>[6x]MAAPARDPPGYRYAAAMVPTGSILSTIEVASHRRLFDFFAAVRSDENSLYDVEFDALLGSYCNTLSLVRFLELGLSVACVCTKFPELAYMNEGRVQFEVHQPLIARDGPHPVEQPVHNYMTKVIDRRALNAAFSLATEAIALLTGEALDGTGISLHRQLRAIQQLARNVQAVLGAFERGTADQMLHVLLEKAPPLALLLPMQRYLDNGRLATRVARATLVAELKRSFCDTSFFLGKAGHRREAIEAWLVDLTTATQPSVAVPRLTHADTRGRPVDGVLVTTAAIKQRLLQSFLKVEDTEADVPVTYGEMVLNGANLVTALVMGKAVRSLDDVGRHLLDMQEEQLEANRETLDELESAPQTTRVRADLVAIGDRLVFLEALEKRIYAATNVPYPLVGAMDLTFVLPLGLFNPAMERFAAHAGDLVPAPGHPEPRAFPPRQLFFWGKDHQVLRLSMENAVGTVCHPSLMNIDAAVGGVNHDPVEAANPYGAYVAAPAGPGADMQQRFLNAWRQRLAHGRVRWVAECQMTAEQFMQPDNANLALELHPAFDFFAGVADVELPGGEVPPAGPGAIQATWRVVNGNLPLALCPVAFRDARGLELGVGRHAMAPATIAAVRGAFEDRSYPAVFYLLQAAIHGNEHVFCALARLVTQCITSYWNNTRCAAFVNDYSLVSYIVTYLGGDLPEECMAVYRDLVAHVEALAQLVDDFTLPGPELGGQAQAELNHLMRDPALLPPLVWDCDGLMRHAALDRHRDCRIDAGGHEPVYAAACNVATADFNRNDGRLLHNTQARAADAADDRPHRPADWTVHHKIYYYVLVPAFSRGRCCTAGVRFDRVYATLQNMVVPEIAPGEECPSDPVTDPAHPLHPANLVANTVKRMFHNGRVVVDGPAMLTLQVLAHNMAERTTALLCSAAPDAGANTASTANMRIFDGALHAGVLLMAPQHLDHTIQNGEYFYVLPVHALFAGADHVANAPNFPPALRDLARHVPLVPPALGANYFSSIRQPVVQHARESAAGENALTYALMAGYFKMSPVALYHQLKTGLHPGFGFTVVRQDRFVTENVLFSERASEAYFLGQLQVARHETGGGVNFTLTQPRGNVDLGVGYTAVAATGTVRNPVTDMGNLPQNFYLGRGAPPLLDNAAAVYLRNAVVAGNRLGPAQPLPVFGCAQVPRRAGMDHGQDAVCEFIATPVATDINYFRRPCNPRGRAAGGVYAGDKEGDVIALMYDHGQSDPARPFAATANPWASQRFSYGDLLYNGAYHLNGASPVLSPCFKFFTAADITAKHRCLERLIVETGSAVSTATAASDVQFKRPPGCRELVEDPCGLFQEAYPITCASDPALLRSARDGEAHARETHFTQYLIYDASPLKGLSL;>[6x]MAAPQFHRPSTITADNVRALGTRGLVLATNNAQFIMDNSYPHPHGTQGAVREFLRGQAAALTDLGVTHANNTFAPQPMFAGDAAAEWLRPSFGLKRTYSPFVVRDPKTPSTP;>MITDCFEADIAIPSGISRPDAAALQRCEGRVVFLPTIRRQLALADVAHESFVSGGVSPDTLGLLLAYRRRFPAVITRVLPTRIVACPVDLGLTHAGTVNLRNTSPVDLCNGDPVSLVPPVFEGQATDVRLESLDLTLRFPVPLPTPLAREIVARLVARGIRDLNPDPRTPGELPDLNVLYYNGARLSLVADVQQLASVNTELRSLVLNMVYSITEGTTLILTLIPRLLALSAQDGYVNALLQMQSVTREAAQLIHPEAPMLMQDGERRLPLYEALVAWLAHAGQLGDILALAPAVRVCTFDGAAVVQSGDMAPVIRYP[2x];> MKTKPLPTAPMAWAESAVETTTSPRELAGHAPLRRVLRPPIARRDGPVLLGDRAPRRTASTMWLLGIDPAESSPGTRATRDDTEQAVDKILRGARRAGGLTVPGAPRYHLTRQVTLTDLCQPNAERAGALLLALRHPTDLPHLARHRAPPGRQTERLAEAWGQLLEASALGSGRAESGCARAGLVSFNFLVAACAAAYDARDAAEAVRAHITTNYGGTRAGARLDRFSECLRAMVHTHVFPHEVMRFFGGLVSWVTQDELASVTAVCSGPQEATHTGHPGRPRSAVTIPACAFVDLDAELCLGGPGAAFLYLVFTYRQCRDQELCCVYVVKSQLPPRGLEAALERLFGRLRITNTIHGAEDMTPPPPNRNVDFPLAVLAASSQSPRCSASQVTNPQFVDRLYRWQPDLRGRPTARTCTYAAFAELGVMPDDSPRCLHRTERFGAVGVPVVILEGVVWRPGGWRACA;> MNAHFANEVQYDLTRDPSSPASLIHVIISSECLAAAGVPLSALVRGRPDGGAAANFRVETQTRAHATGDCTPWRSAFAAYVPADAVGAILAPVIPAHPDLLPRVPSAGGLFVSLPVACDAQGVYDPYTVAALRLAWGPWATCARVLLFSYDELVPPNTRYAADGARLMRLCRHFCRYVARLGAAAPAAATEAAAHLSLGMGESGTPTPQASSVSGGAGPAVVGTPDPPISPEEQLTAPGGDTATAEDVSITQENEEILALVQRAVQDVTRRHPVRARPKHAASGVASGLRQGALVHQAVSGGALGASDAEAVLAGLEPPGGGRFASRGGPRAAGEDVLNDVLTLVPGTAKPR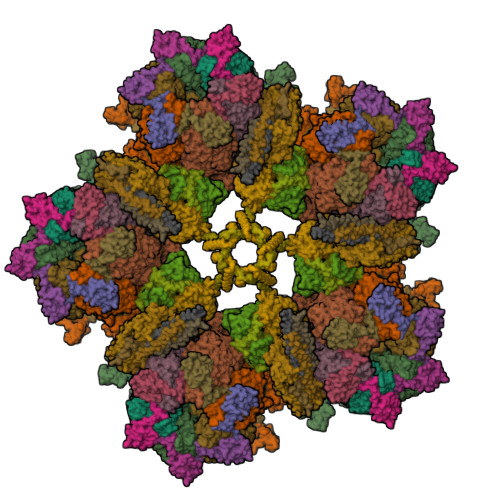SLVEWLDRGWEALAGGDRPDWLWSRRSISVVLRHHYGTKQRFVVVSYENSVAWGGRRARPPRLSSELATALTEACAAERVVRPHQLSPAAQTALLRRFPALEGPLRHPRPVLQPFDIAAEVAFVARIQIACLRALGHSIRAALQGGPRIFQRLRYDFGPHQSEWLGEVTRRFPVLLENLMRALEGTAPDAFFHTAYALAVLAHLGGQGGRGRRRRLVPLSDDIPARFADSDAHYAFDYYSTSGDTLRLTNRPIAVVIDGDVNGREQSKCRFMEGSPSTAPHRVCEQYLPGESYAYLCLGFNRRLCGLVVFPGGFAFTINTAAYLSLADPVARAVGLRFCRGAATGPGLVR;>[2x]MDPYYPFDALDVWEHRRFIVADSRSFITPEFPRDFWMLPVFNIPRETAAERAAVLQAQRTAAAAALENAALQAAELPVDIERRIRPIEQQVHHIADALEALETAAAAAEEADAARDAEARGEGAADGAAPSPTAGPAAAEMEVQIVRNDPPLRYDTNLPVDLLHMVYAGRGAAGSSGVVFGTWYRTIQERTIADFPLTTRSADFRDGRMSKTFMTALVLSLQSCGRLYVGQRHYSAFECAVLCLYLLYRTTHESSPDRDRAPVAFGDLLARLPRYLARLAAVIGDESGRPQYRYRDDKLPKAQFAAAGGRYEHGALATHVVIATLVRHGVLPAAPGDVPRDTSTRVNPDDVAHRDDVNRAAAAFLARGHNLFLWEDQTLLRATANTITALAVLRRLLANGNVYADRLDNRLQLGMLIPGAVPAEAIARGASGLDSGAIKSGDNNLEALCVNYVLPLYQADPTVELTQLFPGLAALCLDAQAGRPLASTRRVVDMSSGARQAALVRLTALELINRTRTNTTPVGEIINAHDALGIQYEQGPGLLAQQARIGLASNTKRFATFNVGSDYDLLYFLCLGFIPQYLSVA;>MIPAALPHPTMKRQGDRDIVVTGVRNQFATDLEPGGSVSCMRSSLSFLSLLFDVGPRDVLSAEAIEGCLVEGGEWTRAAAGSGPPRMCSIIELPNFLEYPAARGGLRCVFSRVYGEVGFFGEPTAGLLETQCPAHTFFAGPWAMRPLSYTLLTIGPLGMGLYRDGDTAYLFDPHGLPAGTPAFIAKVRAGDVYPYLTYYAHDRPKVRWAGAMVFFVPSGPGAVAPADLTAAALHLYGASETYLQDEPFVERRVAITHPLRGEIGGLGALFVGVVPRGDGEGSGPVVPALPAPTHVQTPGADRPPEAPRGASGPPDTPQAGHPNRPPDDVWAAALEGTPPAKPSAPDAAASGPPHAAPPPQTPAGDAAEEAEDLRVLEVGAVPVGRHRARYSTGLPKRRRPTWTPPSSVEDLTSGERPAPKAPPAKAKKKSAPKKKAPVAAEVPASSPTPIAATVPPAPDTPPQSGQGGGDDGPASPSSPSVLETLGARRPPEPPGADLAQLFEVHPNVAATAVRLAARDAALAREVAACSQLTINALRSPYPAHPGLLELCVIFFFERVLAFLIENGARTHTQAGVAGPAAALLDFTLRMLPRKTAVGDFLASTRMSLADVAAHRPLIQHVLDENSQIGRLALAKLVLVARDVIRETDAFYGDLADLDLQLRAAPPANLYARLGEWLLERSRAHPNTLFAPATPTHPEPLLHRIQALAQFARGEEMRVEAEAREMREALDALARGVDSVSQRAGPLTVMPVPAAPGAGGRAPCPPALGPEAIQARLEDVRIQARRAIESAVKEYFHRGAVYSAKALQASDSHDCRFHVASAAVVPMVQLLESLPAFDQHTRDVAQRAALPPPPPLATSPQAILLRDLLQRGQPLDAPEDLAAWLSVLTDAATQGLIERKPLEELARSIHGINDQQARRSSGLAELQRFDALDAALAQQLDSDAAFVPATGPAPYVDGGGLSPEATRMAEDALRQARAMEAAKMTAELAPEARSRLRERAHALEAMLNDARERAKVAHDAREKFLHKLQGVLRPLPDFVGLKACPAVLATLRASLPAGWTDLADAVRGPPPEVTAALRADLWGLLGQYREALEHPTPDTATALAGLHPAFVVVLKTLFADAPETPVLVQFFSDHAPTIAKAVSNAINAGSAAVATASPAATVDAAVRAHGALADAVSALGAAARDPASPLSFLAVLADSAAGYVKATRLALEARGAIDELTTLGSAAADLVVQARRACAQPEGDHAALIDAAARATTAARESLAGHEAGFGGLLHAEGTAGDHSPSGRALQELGKVIGATRRRADELEAAVADLTAKMAAQRARGSSERWAAGVEAALDRVENRAEFDVVELRRLQALAGTHGYNPRDFRKRAEQALAANAEAVTLALDTAFAFNPYTPENQRHPMLPPLAAIHRLGWSAAFHAAAETYADMFRVDAEPLARLLRIAEGLLEMAQAGDGFIDYHEAVGRLADDMTSVPGLRRYVPFFQHGYADYVELRDRLDAIRADVHRALGGVPLDLAAAAEQISAARNDPEATAELVRTGVTLPCPSEDALVACAAALERVDQSPVKNTAYAEYVAFVTRQDTAETKDAVVRAKQQRAEATERVMAGLREALAARERRAQIEAEGLANLKTMLKVVAVPATVAKTLDQARSVAEIADQVEVLLDQTEKTRELDVPAVIWLEHAQRTFETHPLSAARGDGPGPLARHAGRLGALFDTRRRVDALRRSLEEAEAEWDEVWGRFGRVRGGAWKSPEGFRAMHEQLRALQDTTNTVSGLRAQPAYERLSARYQGVLGAKGAERAEAVEELGARVTKHTALCARLRDEVVRRVPWEMNFDALGGLLAEFDAAAADLAPWAVEEFRGARELIQYRMGLYSAYARAGGQTGAGAESAPAPLLVDLRALDARARASSSPEGHEVDPQLLRRRGEAYLRAGGDPGPLVLREAVSALDLPFATSFLAPDGTPLQYALCFPAVTDKLGALLMRPEAACVRPPLPTDVLESAPTVTAMYVLTVVNRLQLALSDAQAANFQLFGRFVRHRQATWGASMDAAAELYVALVATTLTREFGCRWAQLGWASGAAAPRPPPGPRGSQRHCVAFNENDVLVALVAGVPEHIYNFWRLDLVRQHEYMHLTLERAFEDAAESMLFVQRLTPHPDARIRVLPTFLDGGPPTRGLLFGTRLADWRRGKLSETDPLAPWRSALELGTQRRDVPALGKLSPAQALAAVSVLGRMCLPSAALAALWTCMFPDDYTEYDSFDALLAARLESGQTLGPAGGREASLPEAPHALYRPTGQHVAVLAAATHRTPAARVTAMDLVLAAVLLGAPVVVALRNTTAFSRESELELCLTLFDSRPGGPDAALRDVVSSDIETWAVGLLHTDLNPIENACLAAQLPRLSALIAERPLADGPPCLVLVDISMTPVAVLWEAPEPPGPPDVRFVGSEATEELPFVATAGDVLAASAADADPFFARAILGRPFDASLLTGELFPGHPVYQRPLADEAGPSAPTAARDPRDLAGGDGGSGPEDPAAPPARQADPGVLAPTLLTDATTGEPVPPRMWAWIHGLEELASDDAGGPTPNPAPALLPPPATDQSVPTSQYAPRPIGPAATARETRPSVPPQQNTGRVPVAPRDDPRPSPPTPSPPADAALPPPAFSGSAAAFSAAVPRVRRSRRTRAKSRAPRASAPPEGWRPPALPAPVAPVAASARPPDQPPTPESAPPAWVSALPLPPGPASARGAFPAPTLAPIPPPPAEGAVVPGGDRRRGRRQTTAGPSPTPPRGPAAGPPRRLTRPAVASLSASLNSLPSPRDPADHAAAVSAAAAAVPPSPGLAPPTSAVQTSPPPLAPGPVAPSEPLCGWVVPGGPVARRPPPQSPATKPAARTRIRARSVPQPPLPQPPLPQPPLPQPPLPQPPLPQPPLPQPPLPQPPLPQPPLPQPPLPQPPLPPVTRTLTPQSRDSVPTPESPTHTNTHLPVSAVTSWASSLALHVDSAPPPASLLQTLHISSDDEHSDADSLRFSDSDDTEALDPLPPEPHLPPADEPPGPLAADHLQSPHSQFGPLPVQANAVLSRRYVRSTGRSALAVLIRACRRIQQQLQRTRRALFQRSNAVLTSLHHVRMLLG[2x]> GRTCPKPDDLPFSTVVPLKTFYEPGEEITYSCKPGYVSRGGMRKFICPLTGLWPINTLKCTPRVCPFAGILENGAVRYTTFEYPNTISFSCNTGFYLNGADSAKCTEEGKWSPE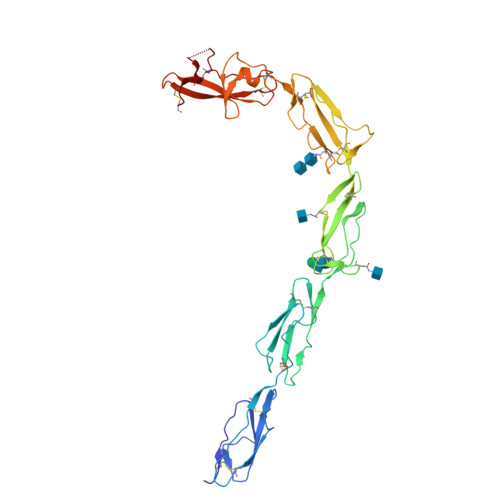LPVCAPIICPPPSIPTFATLRVYKPSAGNNSLYRDTAVFECLPQHAMFGNDTITCTTHGNWTKLPECREVKCPFPSRPDNGFVNYPAKPTLYYKDKATFGCHDGYSLDGPEEIECTKLGNWSAMPSCKASCKVPVKKATVVYQGERVKIQEKFKNGMLHGDKVSFFCKNKEKKCSYTEDAQCIDGTIEVPKCFKEHTDASDVKPC(1R)-2-[(CYANOMETHYL)AMINO]-1-({[2-(DIFLUOROMETHOXY)BENZYL]SULFONYL}METHYL)-2-OXOETHYL MORPHOLINE-4-CARBOXYLATE | C18 H21 F2 N3 O7 S | 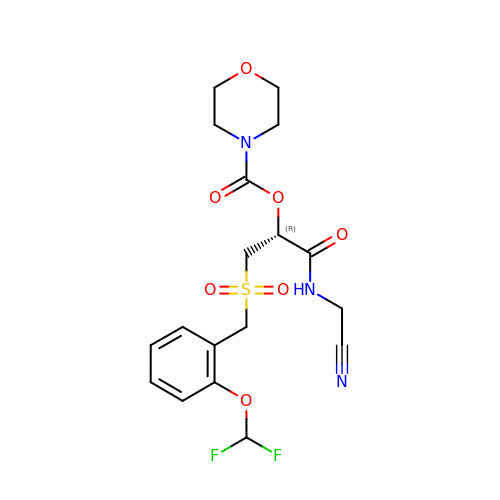YKWHKILAGONYKL-HNNXBMFYSA-N> MSRSKRDNNFYSVEIGDSTFTVLKRYQNLKPIGSGAQGIVCAAYDAILERNVAIKKLSRPFQNQTHAKRAYRELVLMKCVNHKNIIGLLNVFTPQKSLEEFQDVYIVMELMDANL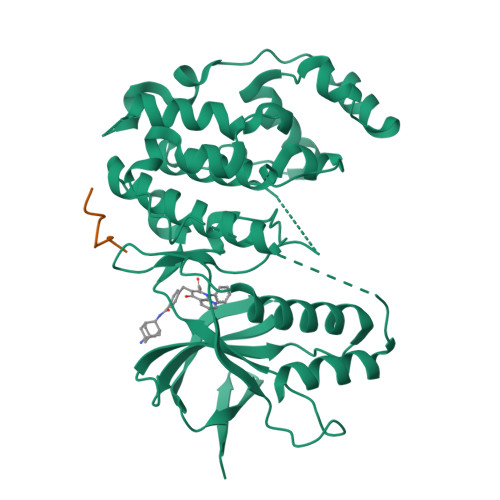CQVIQMELDHERMSYLLYQMLCGIKHLHSAGIIHRDLKPSNIVVKSDCTLKILDFGLARTAGTSFMMTPYVVTRYYRAPEVILGMGYKENVDIWSVGCIMGEMIKGGVLFPGTDHIDQWNKVIEQLGTPCPEFMKKLQPTVRTYVENRPKYAGYSFEKLFPDVLFPADSEHNKLKASQARDLLSKMLVIDASKRISVDEALQHPYINVWYDPSEAEAPPPKIPDKQLDEREHTIEEWKELIYKEVMDLHHHHHH;> KPKRPTTLNLF SEOCALCITOL | 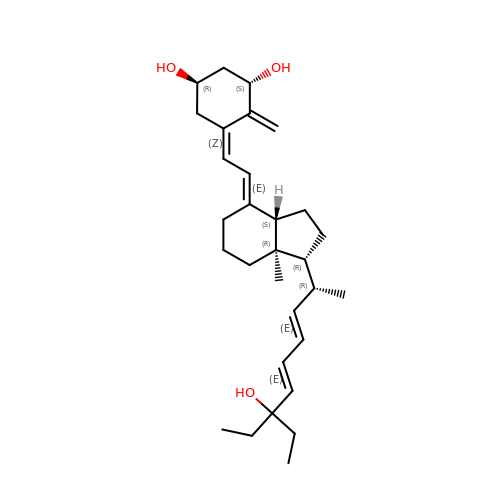C30 H46 O3 | LVLLALCJVJNGQQ-SEODYNFXSA-N> TDLLTKIELQAYNHIRTSETKELQPRIKLINTGNTPITLSEVKIRYYYTKDQVINEIYTCDWSN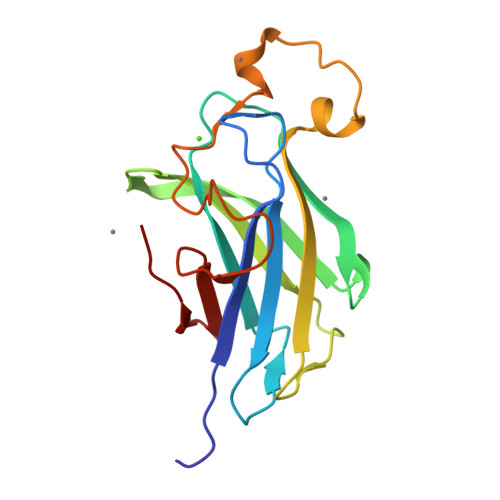ITSSKITGTVVQMSNPKPNADSYVEIGFTNSAGVLNPGEYVEIISRIGNSYALSLATPPYSEWNYMYDQNSDYSFNNSSSDFVVWDKITVYISGTLYWGIEP>[4x]SAKILAIDTATENCSVALLVNDQVISRSEVAPRDHTKKVLPMVDEVLKEAGLTLQDLDALAFGRGPGSFTGVRIGIGIAQGLAFGAELPMIGVSTLAAMAQASYRLHGATDVAVAIDARMSEVYWARYSRQENGEWIGVDEECVIPPARLAEEAQADSKTWTTAGTGWSAYQEELAGLPFNTADSEVLYPDSQDIVILAKQELEKGNTVPVEE

The yeaZ gene product forms part of the conserved network YjeE/YeaZ/YgjD essential for survival of many eubacteria. [3] and V. parahaemolyticus (C. Thomas, personal communication, 19 November 2010) demonstrated that among other as yet unidentified roles, YeaZ functions as a resuscitation promoting factor required for cells to be able to survive in, and exit from, a VBNC state. The structure of VpYeaZ confirmed that it is a member of the ASKHA superfamily of actin-like nucleotide-binding proteins characterized by two domains (I and II) that hold a nucleotide-binding site in the interdomain cleft. EcYeaZ has been shown to interact with the conserved essential proteins YjeE and YgjD, with YgjD being the preferred interaction partner.

In this paper, we report the crystal structure of V. parahaemolyticus YeaZ (VpYeaZ) to 3.1 Å resolution. The structure of VpYeaZ has been solved to 3.1 Å resolution revealing a two domain architecture with a duplicated βββαβαβα secondary structure. The asymmetric unit contains four subunits, each comprising residues 2–213. The 19 C-terminal residues are missing, most likely having been proteolytically removed during crystallization. Remarkably, YeaZ appears to be unique amongst other members of ASKHA superfamily in that it lacks these inserts; the lengths of loops β3α1, β4α2, α2β5 and β3′α1′ in VpYeaZ do not exceed five residues. Analysis of the packing of VpYeaZ monomers in the crystal lattice identified an obvious dimer with 2-fold symmetry and approximate dimensions of 30×45×80 Å. The dimer interface is formed by residues from helices α1 and α2 from both subunits, which form a 4-helical bundle. The dimer interface in this form shields 9–10% of the monomer surface area and buries a region of strongly conserved hydrophobic residues L40, L47, I74, I78, L82 (VpYeaZ numbering).>MKYRCKVCDYIYDPEVGDPTSGIKPGTPFQELPEDWLCPVCNVGKDQFEPLRGEVRRVRPEDIDMFCYQCSQTVRGRACTVKGVCGKEATVARLQDNLLFAIKGISAYLYHARELGYTDEVVDAFLERGFYSTLTNVNFDAEEFVSLALEAGEMNLRTMKLLKKAHMDTYGEPEPAEVRVGALDGPAIIATGHSLKALEELLKQTEGSGVNVYTHSELLPAHGYPGLRKYPHLAGQLGGPWFDQRETFSRYSAAVLGTSNCVLLPRDSYRDRMFTCGVARLPGVEHVDGYDFSPVIEKALELPPLKEEDSATLTTGFGLSTILSLADKIKELVEEGKIRRFFLVGGCD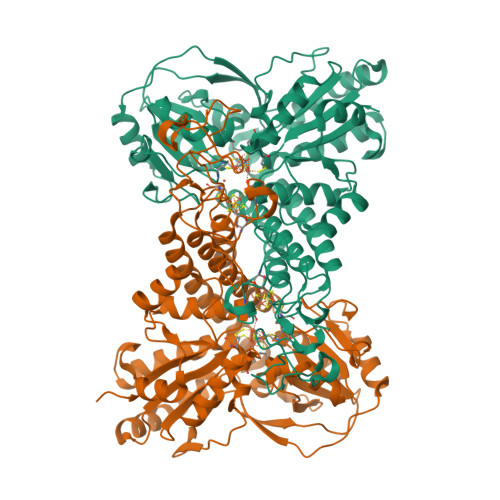SPLPQAKYYTEFVRKLPEDTVVLTLACGKYRFNSMDLGDIDGIPRLIDLGQCNDSIVAVELVEALSNLFSMDVNELPLSIVLSWMEQKAAAILWSLLSLNLRGMYIGPILPGWANDDIINVLVDKYELTPIGDPEEDIKKMMEVDKLAAALEHHHHHH[4x]> AQSVPYGVSQIKAPALHSQGYTGSNVKVAVIDSGIDSSHPDLKVAGGASMVPSETNPFQDNNSHGTHVAGTVAALNNSIGVLGVAPSASLYAVKVLGADGSGQYSWIINGIEWAIANNMDVINMSLGGPSGSAALKAAVDKAVASGVVVVAAAGNEGTSGSSSTVGYPGKYPSVIAVGAVDSSNQRASFSSVGPELDVMAPGVSIQSTLPGNKYGAYNGTSMASPHVAGAAALILSKHPNWTNTQVRSSLQ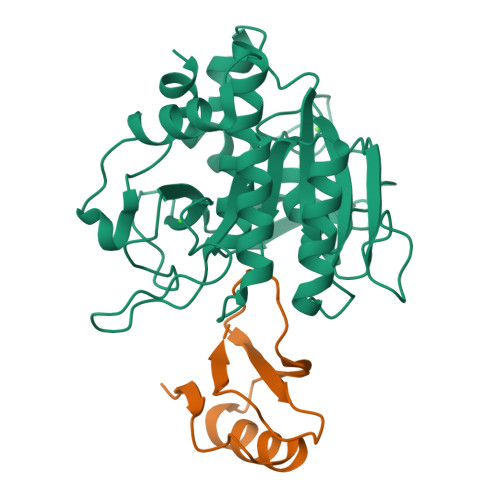NTTTKLGDSFYYGKGLINVQAAAQ;> SSVEKKPEGVNTGAGDRHNLKTEWPELVGKSVEEAKKVILQDKPEAQIIVLPVGTIVTMEYRIDRVRLFVDKLDNIAEVPRVG>DKATIPSESPFAAAEVADGAIVVDIAKMKYETPELHVKVGDTVTWINREAMPHNVHFVAGVLGEAA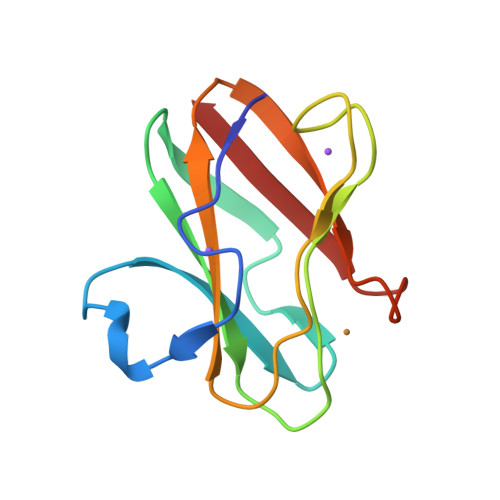LKGPMMKKEQAYSLTFTEAGTYDYHCTPHGFMRGKVVVE[4x]> MEILYTGASESLHSTILKALLERIDLGDTFISDNYTRWQATERYYMMYKIPNKKDKAAIEKWNKGDTDFKSLVMPYSYAQLMTAHAYMVNVFLNRDPIFQTDSLNGDGTERELALESMLQYQVKAGEMEPSLLVWFMDALRYGVGVLGDYWEEHVFHQTVFEVK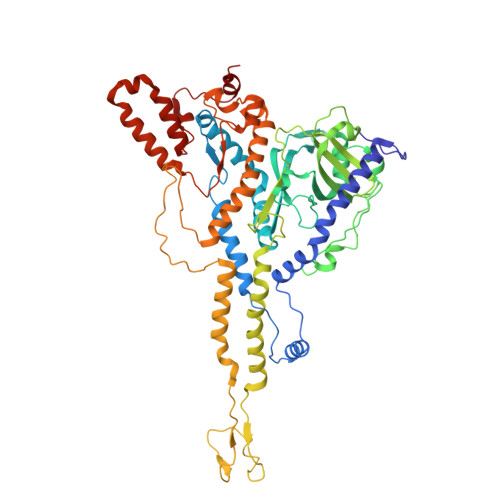KTRVVKGYEGCKTFNVMVYDFIPDPRVALCKYQEGEFFGRRLDLNVLDLKKGAKFGKYFNVEHAEALVAASKEEMYRRDPSIGQQRSLKDSTMTPKGKQVGDISCVEIFVRLVPKDWGLGDSEFPEMWVFTVADKKYIVAAEPVNTLDDKFPFHILECEIDGYMNKSRGLLEISAPMNDILTWLFDSHMYNKRQIMNNQFIGDPSALVVKDVESKEPGKFIRLRPIISQLPVTDVTAQNIQDVQVVERNMQRIVGVNDDVAGQSSPSSRRSATEFRGTTSFASSRLANLAYFFSVTGFRSLAKSLIVKTQQLYTVEMKVKVAGDNIKGAQSIIVKPEDISGQFDIMPVDGTLPVDRMAQAQFWMQIMSMVAGNPVLGAEYRLGDIFSYTARLAGLKGIDKMKIRILDDDQILALILA>MIRTGKQYLESLNDGRNVWVGNEKIDNVATHPKTRDYAQRHADFYDLHHRPDLQDV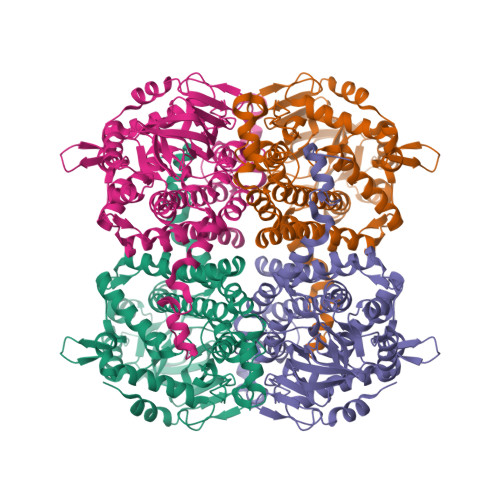MTFVDKDGERRTMQWFGHYDKEQLRRKRKYHETIMREMAGASFPRTPDVNNYVLQTYIDDPSPWETQTIGAEGKVKAKNIVDFVNFAKKHDLNCAPQFVDPQMDRSNPDAQQRSPGLRVIEKNDKGIVVSGVKAIGTGVAFADWIHIGVFFRPGIPGDQIIFAATPVNTPGVTIVCRESVVKEDPIEHPLASQGDELDGMTVFDNVFIPWSHVFHLGNPEHAKLYPQRVFDWLHYHALIRQSVRAELMAGLAILITEHIGTNKIPAVQTRVAKLIGFHQAMLAHIVASEELGFHTPGGAYKPNILIYDFGRALYLENFSQMIYELVDLSGRSALIFASEDQWNDEALNGWFERMNNGPVGQPHDRVKIGRVIRDLFLTDWGNRLFVFENFNGTPLQAIRMLTMQRAEFSAAGPYGTLARKVCGIELTEGHDSEYKATAGYAQALDSARHQEKLALSGTMTV[4x]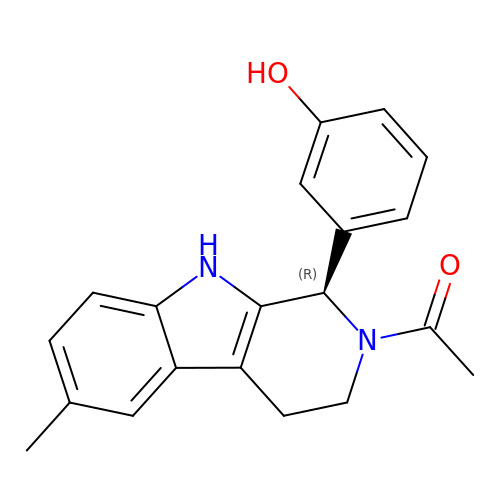3-[(1R)-2-acetyl-6-methyl-2,3,4,9-tetrahydro-1H-beta-carbolin-1-yl]phenol | C20 H20 N2 O2 | ZNGGYWGHJZJJDR-HXUWFJFHSA-N>[3x]GPGSLSQASADLEATLRHKLTVMYSQINGASRALDDVRNRQQDVRMTANRKVEQLQQEYTEMKALLDASETTSTRKIKEEEKRVNSKFDTIYQILLKKKSEI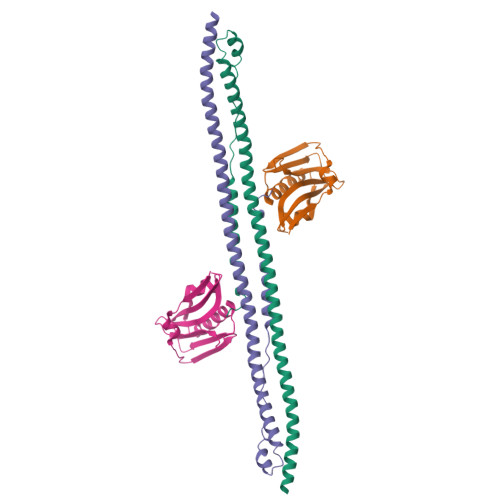QTLKEEIEQSLTKRDEFEFLEKASKLRGISTKPVYIPEVELNHKLIKGIHQSTIDLKNELKQCIGRLQELTPSSGDPGEHDPASTHKSTRP;>[3x]GPGTMASVPASRYLTDMTLEEMSREWSMLIPKQKVAGPLCIRMDQAIMDKNIILKANFSVIFDRLETLILLRAFTEEGAIVGEISPLPSLPGHTAEDVKNAVGVLIGGLEWNDNTVRVSETLQRFAWRSSNENGRPPLTPKQKREMAGTIRSEV>[2x]M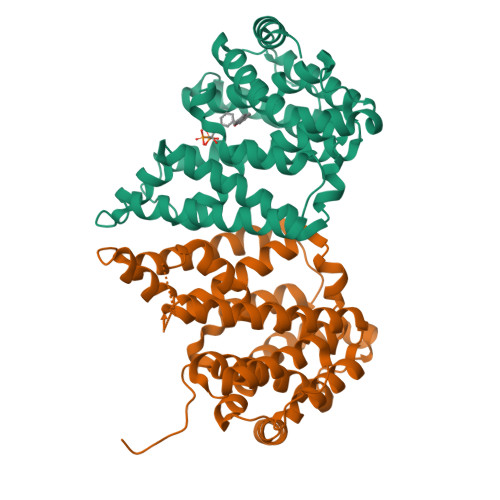IQTERAVQQVLEWGRSLTGFADEHAVEAVRGGQYILQRIHPSLRGTSARTGRDPQDETLIVTFYRELALLFWLDDCNDLGLISPEQLAAVEQALGQGVPCALPGFEGCAVLRASLATLAYDRRDYAQLLDDTRCYSAALRAGHAQAVAAERWSYAEYLHNGIDSIAYANVFCCLSLLWGLDMATLRARPAFRQVLRLISAIGRLQNDLHGCDKDRSAGEADNAVILLLQRYPAMPVVEFLNDELAGHTRMLHRVMAEERFPAPWGPLIEAMAAIRVQYYRTSTSRYRSDAVRGGQRAPA>AECKVTVDSTDQMSFNTKDIAIDKSCKTFTVELTHSGSLPKNVMGHNLVISKEADMQPIATDGLSAGIDKQYLKDGDARVIAHTKVIGAGEKDSV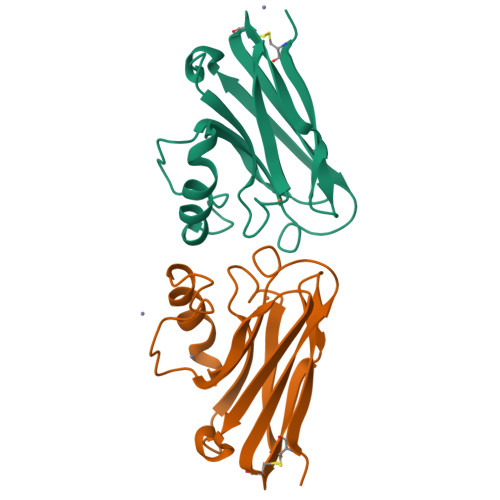TFDVSKLAAGEKYGFFCSFPGHISMMKGTVTLK[2x]> SMVSLGHLAKGASLDDLIDSCIQSFDADGNLCRSNQLLQVMLTMHRIVISSAELLQKVITLYKDALAKNSPGLCLKICYFVRYWITEFWVMFKMDASLTDTMEEFQELVKAKGEELHCRLIDTTQINARDWSRKLTQRIKSNTSKKRKVSLLFDHLEPEELSEHLTYLEFKSFRRISFSDYQNYLVNSCVKENPTMERSIALCNGISQWVQLMVLSRPTPQLRAEVFIKFIQVAQKLHQLQNFNTLMAVIGGLCHSSISRLKETSSHVPHEINKVLGEMTELLSSSRNYDNYRRAYGECTDFKIPILGVHLKDLISLYEAMPDYLEDGKVNVHKLLALYNHISELVQLQEVAPPLEANKDLVHLLTLSLDLYYTEDEIYELSYAREPRNHRAPPLTPSKPPVVVDWASGVSPKPDPKTISKHVQRMVDSVFKNYDHDQDGYISQEEFEKIAASFPFSFCVMDKDREGLISRDEITAYFMRASSIYSKLGLGFPHNFQETTYLKPTFCDNCAGFLWGVIKQGYRCKDCGMNCHKQCKDLVVFECKKRAKNPVAPTENNTS

An intriguing aspect of lymphocyte development is that the generation of a population of self-tolerant immune cells requires Ras activation by two distinct guanine nucleotide exchange factors, Ras guanine nucleotide releasing protein 1 (RasGRP1) and Son-of-Sevenless (SOS). To identify the structural basis for the regulation of RasGRP1, we have determined two crystal structures of RasGRP1. RasGRP1 is maintained in an autoinhibited, dimeric state, which is released by the coordinated binding of diacylglycerol and calcium second messenger molecules.

We determined a crystal structure of RasGRP1CEC at 3.0 Å resolution. The first structure includes the REM, Cdc25, EF and C1 domains and suggests a structural basis for autoinhibition by the regulatory domains. In contrast, the RasGRP1 helical hairpin (residues 355–398) in the absence of Ras is rotated ∼15° away from the active site with respect to its orientation in active SOS, which is consistent with an open conformation that is poised to bind to Ras. The regulatory module of RasGRP1, containing the EF and C1 domains, interacts extensively with the Cdc25 domain. Metal ions are not present in either EF hand in the crystal structure. An electron density map calculated with phases derived from the model for the four domains of RasGRP1CEC reveals additional electron density for a peptide traversing the Ras binding site in the Cdc25 domain. This electron density can be assigned unambiguously to a portion of the linker between the Cdc25 and EF domains, but strong electron density is present only for the central eight residues of the linker. The visible portion of the linker shows that several residues, including Val 450, Val 452 and Trp 454, dock within a hydrophobic groove at the base of the RasGRP1 helical hairpin. Clearly, occupation of this site on the Cdc25 domain by the Cdc25-EF linker will prevent Ras binding and nucleotide exchange. An extensive dimer interface is generated at a twofold symmetry axis in the crystal, burying ∼2500 Å2 of surface area between the two subunits in the dimer.[(2~{R},3~{S},4~{R},5~{R})-5-(6-aminopurin-9-yl)-3,4-bis(oxidanyl)oxolan-2-yl]methoxy-~{N}-[(2~{S})-1-methoxy-1-oxidanylidene-propan-2-yl]phosphonamidic 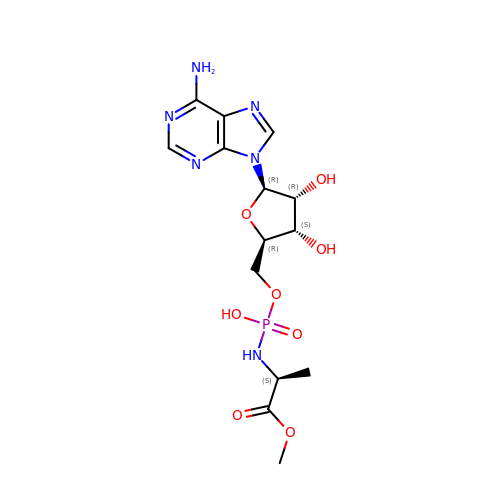acid | C14 H21 N6 O8 P | KHSIAISBDZSYJB-WFMPWKQPSA-N>[2x]MENLIGYVAAFLTTVSFLPQVLRVVMTKQTRDISRNMYIMFFLGVV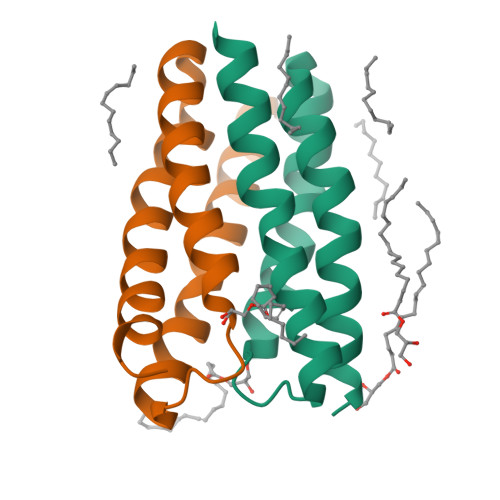LWFVYGILRSDLPIILANVVTLFFVTIILYYKLTEGNQTGSLEVLFQ>[2x]GSGSGDVMRR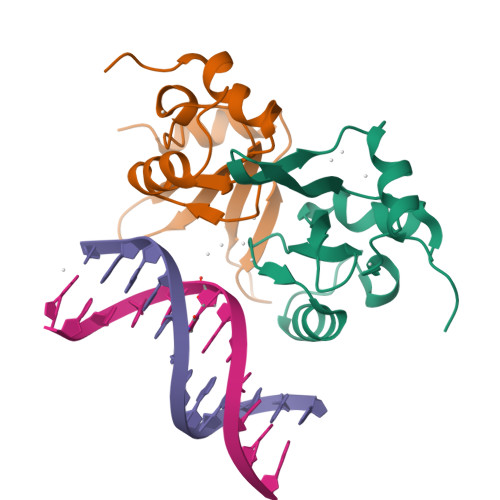RIATPEEVRLPLQHGWRREVRIKKGSHRWQGETWYYGPCGKRMKQFPEVIKYLSRNVVHSVRREHFSFSPRMPVGDFFEERDTPEGLQWVQLSAEEIPSRIQAITGKRG(4-tert-butylphenyl)acetaldehyde 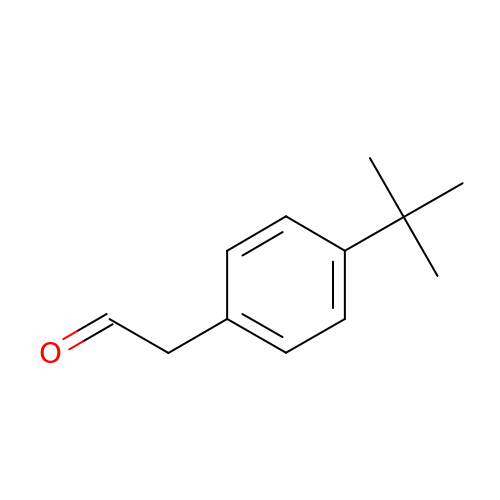| C12 H16 O | VMLYBYNXKMHLIJ-UHFFFAOYSA-N> MGKTNDWLDFDQLA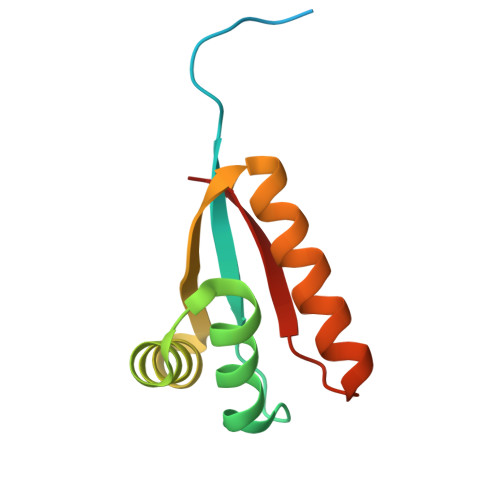EEKVRDALKPPSMYKVILVNDDYTPMEFVIDVLQKFFSYDVERATQLMLAVHYQGKAICGVFTAEVAETKVAMVNKYARENEHPLLCTLEKAF>[2x]AMNEAGQKKTDKDRVLSLDAATIVGEQQDETTYNVDRSASKKYTAPLLDTPRSVTVVPKQVIKDTAAVSLQDALRTVPGITFGAGEGGNPTGDRPFIRGFDAQSDTYVDGVRDTGAQTREIFNLEQIEVSKGPNSAFGGRGSAGGSLNLVSKQAKAGNFIDGGFTYGSDQTRRYTLDLNQEFLDGNAAFRLNLLKHDANVAGRDEVDVSRWGVAPSLTFGLGSPTRVTVSHYHLESDDTPDSGIPYAKSSDRSKHNPDKPVNVDRGNFYGLTGRDFQKSRIDTSTITVEHDLTDSLTIRNTSRYGNSHQDYLWTQPDDSQGNINNGSVWRRQNNRVSTTTTAVNQTDLFGEFYLGGFKNSFSTGLEFSREDSKRDGYIVDTNTGLGSNKCNPSLIGAPSGYNCTSLENPNPHDPWNGSITRKYAPLNTVGTTKAIYAFDTIDLNEQWQVNIGARFDSFETTAKNHGVRPATKLSDKSSFWNWQAGLVW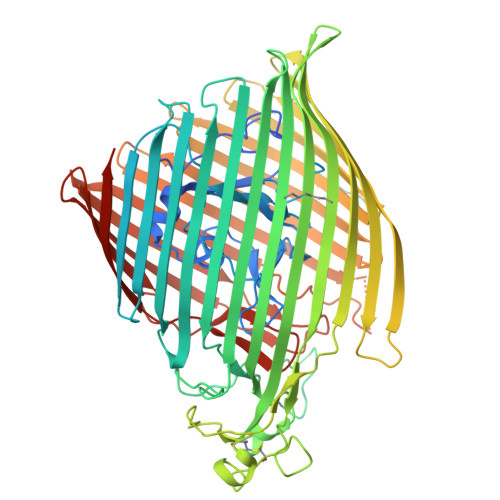KPVPNGSIYASYATSATPPGSMLDNGDTSNAVDGFAISNNLEPEETTNYELGTKWAFFNERLELSAAIFRTDKDNTRILVANQTYDNAGQSRVDGVELSASGKLTEKWKVFAGYSYLDSELVDAGKAGRNGNVNASAASNNGNEMPNTPKNSFSLWTTYDIFPKTTIGGGAFYVDKVYGDVGNTVYVPDYWRYDAMASYKLSKNVDFQLNVQNVFDKKYFDKAYAAHYASQAAGRTILFSTNFHFLEHHHHHH> MYYSSSKPIKKKPNTGISEFNPTQSQIQQQSCNYKITPTYDLPFILTQAINDENQQHQIEQDLTGSLSSRDGTCFIIYSNELFIWTIDKPQYCDRIELPIKQNITRQHIVVYKNKSSSERFSVFLCSPLTGYIRFWGNSSKPNVSQDLPLENPGNNNNFKIFITECQPFGVIVGNSLGSIYLVSVKNNNNLISKKINKSQGMLSYLYLSRQSPVISVFSSPINQQQLQNNNNSHHHHHHHSTTLSSNNFSTIPSRFIYILTEGSLLKYEIENGTERIILDFPIQKEITKLFSNFPKFHQMNIDTIIDQNKDEIQIVNFILYETSASQNLVKYYILQIEIQDDQVLRIKRLDSFSANKKLGGGVTSIEPILQTNSLKYYLTWFDNIYYYSNGGGGGGGVNGIISGSISFQSDIAFSGFYKNQFYFFSEQGINKLDIQPFGSGQLASSELHIQDTIKNIESDIYMDTDNTTSVTGTPATTASATISTTPTIVSPILFDIPKDENLIGSKRNNVLKLMNSFSLKQHTRVDQFVKICKGYNDFDQVIQQVSLWIIDQQPNSKFWAEDGKLLHMFVKEISVQLNQQLEDKKKRHNFLLTCIKDTDLDKLLTTQTKEILKKNEIKIKCAIELRNYQNQQEQSRKSLNYTTTTTTIMKGASSSSSIFSQLIESLVAERNPNWTNIGMNVFELFYSNVSGIDQILINITSKLQELLQNQPQQQQLLTSANKAQILLENCELFYLISSSFPVEYLNSPIIQSTSISIHNLFPKVIQSILNFIQLEFPNQVAGLLGGGGIGGLGNGHSSSSSTILFKKDLGIPNVDKQLYDHLYKLTEKYLYSLKINQFEQFNQFKTKLIEPFVECFKFQEAITLANQFDDFFTLINVYCYQQHQLQNSTITIATTITPADNNKLLIDCLNKFEKIGQLSKVYEYMLERDLKSELLQLPSDFNDSLFRFLQSNSELSWIHSIRMKNWTNVSNTLYQKSISNQHHQQQQQQQQHQVMTLKEKQKLLSLSKVSLMVSTATSSSSSSSSLELQLQPSQQIQLDVINQNLSLIKSQKFFLPDLKNVLSVSEVVQLILQREIGDEDPMVNFVSC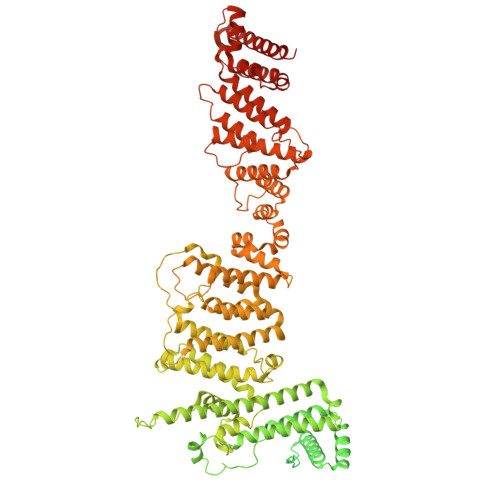IEIISESPLLLKKEEVKELLKLILELSIVNETVFFEKSISDIQLSYSLKETKFYNLISHPHFPKEIALVLLSPIIEDFYKTHINSNKFSSLDDKRQFEISVARLLELSKLEIGQKQI> AADTAPADSLYS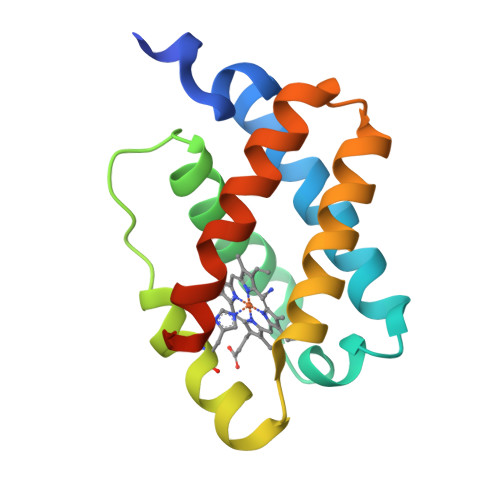RMGGEAAVEKAVDVFYERIVADPQLAPFFANVDMKKQRRKQVAFMTYVFGGSGAYEGRDLGASHRRLIREQGMNHHHFDLVAAHLDSTLQELGVAQELKAEAMAIVASARPLIFGTGEAGAAN>TTCVVVRKGDEVAIGADALVTFGDTRLSRAYERNQKVIPVGDSFVGLAGTTAHFPVMRSLLTGMGEECRLHTRDDVFRTFLKVHEKLKNEYFINTKEDEDDPYESSQIVCLIANSGGIFGVYSYREVFSFDRFWGIGSGRNYALGAMHAVYDRTDLDAGAIARIGVEAGIEFDKSSAAPIDVHTVRLQVATNKDGAA[2x]

The second hitherto unknown bacterial proteasome family member was primarily found in Betaproteobacteria, hence its name BPH, short for Betaproteobacterial proteasome homologue. In this study, we present the first experimental characterization of two bacterial BPH proteins. Their crystal structures reveal homo-oligomeric double-barrel complexes with internalized active sites akin to those of proteasome and HslV. Unique structural features, however, like an elongated inner pore loop with a highly acidic sequence, distinguish BPH from its relatives. Confirming an initial hypothesis, our cluster analysis shows that BPH branches off from HslV and appears to be its direct descendant.

In contrast to the Td-BPH crystals, the obtained Cm-BPH crystal form was not compatible with an assembly of 7-fold symmetry. The data could be scaled to 2.1 Å in space group P6, with unit cell dimensions suggesting two monomers in the ASU. Via the 6-fold symmetry, they form a dodecameric double ring with intersubunit interfaces reminiscent of the tetradecameric Td-BPH but resembling the architecture of dodecameric HslV. A closer inspection of the Cm-BPH crystal structure reveals two malonate molecules from the crystallization buffer to be bound per Cm-BPH protomer, specifically intercalated into the intersubunit clefts of the rings from the outside. Like wedges, they bridge a part of the native intersubunit interactions formed in the Td-BPH rings, thereby leading to an increased curvature favoring hexameric rings. These hexamers are presumably stabilized in the crystallization process, allowing for the tight crystal packing depicted in Fig. S5. A potential result of the smaller radius is a different conformation of the pore loop as compared with the Td-BPH structure. The smaller radius allows for a tighter interaction between neighboring pore loops within the rings. In contrast to Td-BPH, the pore loops are fully ordered, although this presumably represents a non-physiological conformation. The apparent ability of Cm-BPH to assemble into closed rings of ancestral symmetry, albeit artificially stabilized by intercalating malonate molecules in a rigid crystal packing, demonstrates how small structural changes (mimicked by the malonate) can affect the oligomerization symmetry within the proteasome family.>[2x]MLYKELGRTGEEIPALGLGTWGIGGFETPDYSRDEEMVELLKTAIKMGYTHIDTAEYYGGGHTEELIGKAIKDFRREDLFIVSKVWPTHLRRDDLLRSLENTLKRLDTDYVDLYLIHWPNPEIPLEETLSAMAEGVRQGLIRYIGVSNFDRRLLEEAISKSQEPIVCDQVKYNIEDRDPERDGLLEFCQKNGVTLVAYSPLRRTLLSEKTKRTLEEIAKNHGATIYQIMLAWLLAKPNVVAIPKAGRV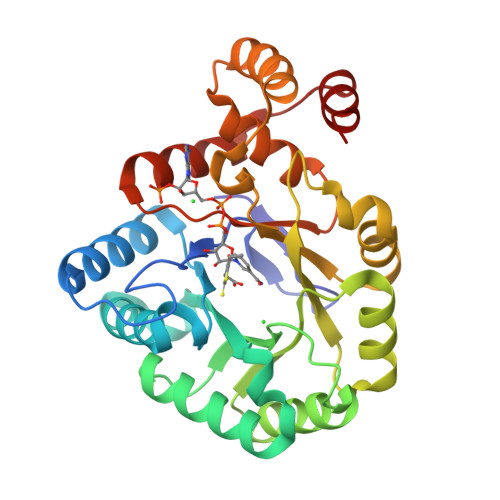EHLRENLKATEIKLSEEEMKLLDSLG>VRSSSRTPSDMPVAHVVANPQAEGQLQWLNRRANALLANGVELRDNQLVVPSEGLYLIYSQVLFSGQGCPSTHVLLTHTISRIAVSYQTPVNLLSAIRSPCQRETPEGAEANPWYEPIYLGGVFQLEPGDRLSAEINRPDYLDFAESGQVYFGIIAL[6x];>[6x]APEPG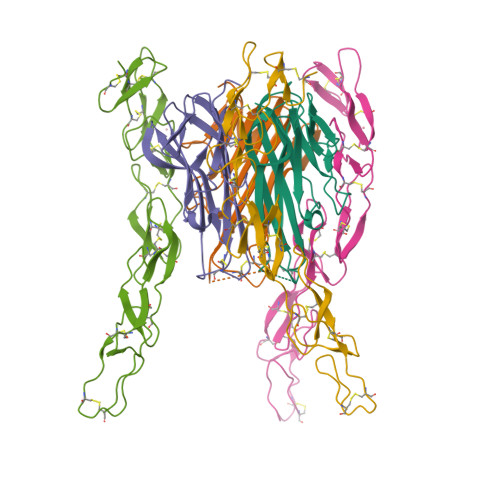STCRLREYYDQTAQMCCSKCSPGQHAKVFCTKTSDTVCDSCEDSTYTQLWNWVPECLSCGSRCSSDQVETQACTREQNRICTCRPGWYCALSKQEGCRLCAPLRKCRPGFGVARPGTETSDVVCKPCAPGTFSNTTSSTDICRPHQICNVVAIPGNASMDAVCTSTSP> NTKYNKEFLLYLAGFVDGDGSIIAQIKPRASNKFAHQLSLTFAVTQKTQRRWFLDKLVDEIGVGYVYDSGSVSDYRLSEIKPLHNFLTQL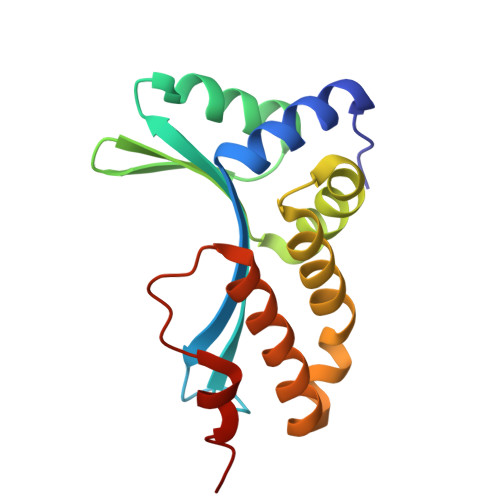QPFLKLKQKQANLVLAIIEQLPSAKASPDAFLEVCTWVDQIAALNDSKTRATTSATVRAALD>MFHILRLESTVDLSEPLKDNGIIVFQSDKLDLEPSPNLGPTGIDNTNVNLINAKGDVLLHIGIRRRENAFVFNSIPYGESRGPEERIPLEGTFGDRRDPSITIFDHPDRYQIMIDYKTVYYYKKRLEGRCEKVSYKINEGQTPPFSDVLGV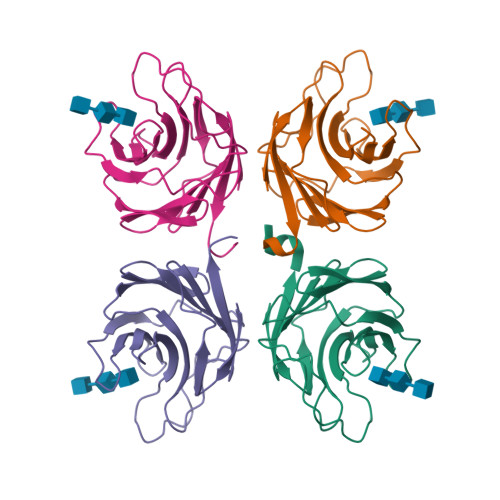TVLYFANVMPRAN[4x]5-(HYDROXYMETHYL)-8-(1H-PYRROL-2-YL)-2H-[1,2,4]TRIAZOLO[4,3-A]QUINOLIN-1-ONE | C15 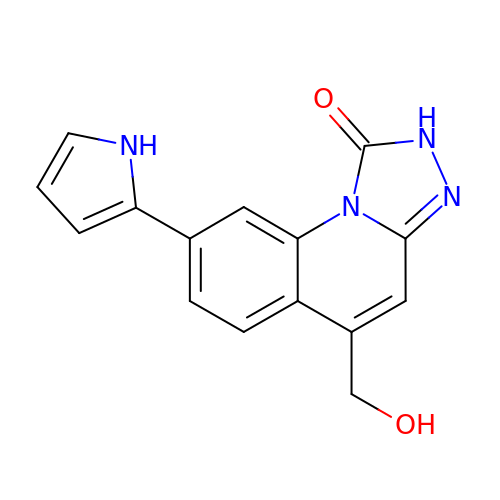H12 N4 O2 | FEKDFTQZRBQDGS-UHFFFAOYSA-N>[24x]VESSTDGQVVPQEVLNLPLEKAHEEADDYLDHLLDSLEELSEAHPDCIPDVELSH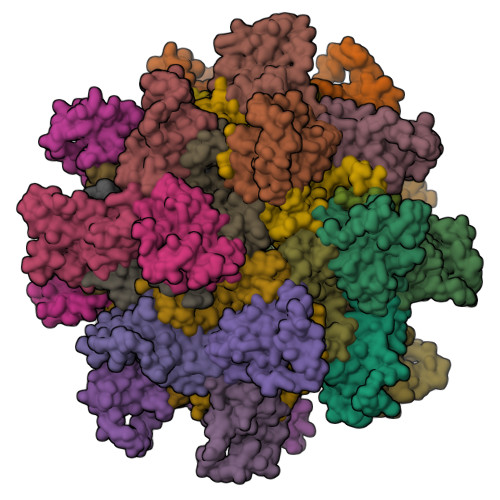GVMTLEIPAFGTYVINKQPPNKQIWLASPLSGPNRFDLLNGEWVSLRNGTKLTDILTEEVEKAISK;>[24x]GSHMSSITKRLYHPKVIEHYTHPRNVGSLDKKLPNVGTGLVGAPACGDVMRLQIKVNDSTGVIEDVKFKTFGCGSAIASSSYMTELVQGMTLDDAAKIKNTEIAKELSLPPVKLHCSMLAEDAIKAAIKDYKSKRNTPTMLS> MIALIQRVSQAKVDVKGETIGKIGKGLLV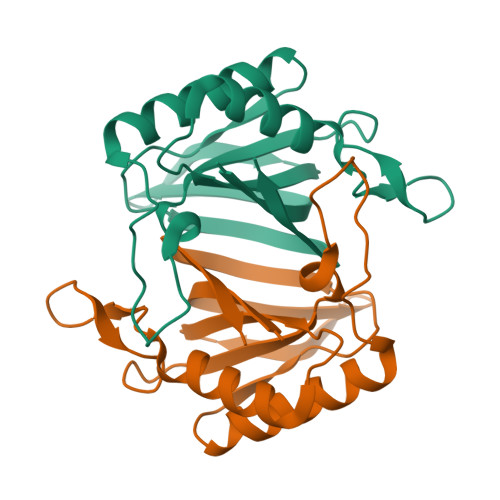LLGVEKEDNREKADKLAEKVLNYRIFSDENDKMNLNVQQAQGELLIVSQFTLAADTQKGLRPSFSKGASPALANELYEYFIQKCAEKLPVSTGQFAADMQVSLTNDGPVTFWLNV For bc1 complex (complex III) assembly, the iron–sulfur protein Rip1 must first be imported into the mitochondrial matrix to fold and acquire its 2Fe–2S cluster, then translocated and inserted into the inner mitochondrial membrane (IM). This translocation of folded Rip1 is accomplished by Bcs1, an unusual heptameric AAA ATPase that couples ATP hydrolysis to translocation. Here, contrary to most AAA-ATPases that form hexameric rings with rather narrow central pores, Bcs1 was shown to form heptameric rings with a significantly wider pore and two large vestibules. One protomer consists of three domains, a transmembrane helix (TMH) at the N-terminus, a Bcs1-specific β-sheet-containing middle domain and a C-terminal AAA cassette.

In addition, no ADP density was found in the ATP-binding pocket of any of the seven protomers (Fig. EV2A,B). Rip1-FeS introduces asymmetry in the matrix vestibule by exclusively contacting the AAA domains of four Bcs1 protomers, henceforth called protomers A–D. It binds to Bcs1 with the 2Fe–2S cluster binding subdomain (FeSD) tightly packing against protomers C and D while the large (base) domain (BD) is exposed to protomers A and B. Based on resolved secondary structure including several side chains in the Rip1-FeS density (left panel and Fig. EV3), we could position the FeS domain with its N- and C-termini facing towards the seal pore locking up the IM vestibule. In this orientation, the N-terminal TM helix would also face towards the IM vestibule. In Bcs1, we identified two highly conserved charged motifs, the EWR motif (E212-R214) and the DDR motif (D300-R302), that contain residues exposed to the FeS domain of Rip1. Second, the EWR and DDR motifs—together with F209—formed a module that contributes to substrate contacts in all four interacting protomers. Thereby, a characteristic positive charge distribution pattern is established in the matrix vestibule that is complementary to several negatively charged residues, e.g., D139, D145, E201 and D210 in the Rieske substrate. Indeed, we found that Bcs1 charge inversion mutations in the EWR and the DDR motives were not viable in YP medium containing glycerol.

>[7x]MGKHHHHHHGGGDYKDDDDKGSGHMSDKPIDIQYDKQATPNLSGVITPPTNETGNDSVREKLSKLVGDAMSNNPYFAAGGGLMILGTGLAVARSGIIKASRVLYRQMIVDLEIQSKDKSYAWFLTWMAKHPQRVSRHLSVRTNYIQHDNGSVSTKFSLVPGPGNHWIRYKGAFILIKRERSAKMIDIANGSPFETVTLTTLYRDKHLFDDILNEAKDIALKTTEGKTVIYTSFGPEWRKFGQPKAKRMLPSVILDSGIKEGILDDVYDFMKNGKWYSDRGIPYRRGYLLYGPPGSGKTSFIQALAGELDYNICILNLSENNLTDDRLNHLMNNMPERSILLLEDIDAAFNKRSQTGEQGFHSSVTFSGLLNALDGVTSSEETITFMTTNHPEKLDAAIMRPGRIDYKVFVGNATPYQVEKMFMKFYPGETDICKKFVNSVKELDITVSTAQLQGLFVMNKDAPHDALKMVSSLRNANHIF;> AKVEVNLAAIPLGKNVVVKWQGKPVFIRHRTPHEIQEANSVDMSALKDPQTDADRVKDPQWLIMLGICTHLGCVPIGEAGDFGGWFCPCHGSHYDISGRIRKGPAPLNLEIPAYEFDGDKVIVG>MIPAHVPADRVVDFDIFNPPGVEQDYFAAWKTLLDGPGLVWSTANGGHWIAARGDVVRELWGDAERLSSQCLAVTPGLGKVMQFIPLQQDGAEHKAFRTPVMKGLASRFVVALEPKVQAVARKLMESLR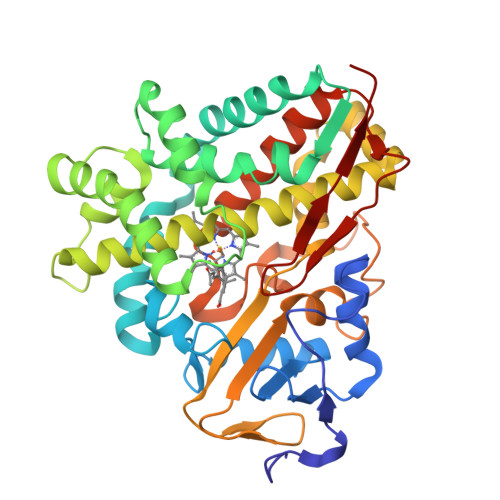PRGSCDFVSDFAEILPLNIFLTLIDVPLEDRPRLRQLGVQLTRPDGSMTVEQLKQAADDYLWPFIEKRMAQPGDDLFSRILSEPVGGRPWTVDEARRMCRNLLFGGLDTVAAMIGMVALHLARHPEDQRLLRERPDLIPAAADELMRRYPTVAVSRNAVADVDADGVTIRKGDLVYLPSVLHNLDPASFEAPEEVRFDRGLAPIRHTTMGVGAHRCVGAGLARMEVIVFLREWLGGMPEFALAPDKAVTMKGGNVGACTALPLVWRA[6x]>[2x]MPNKYIVVTGGVLSSVGKGTLVASI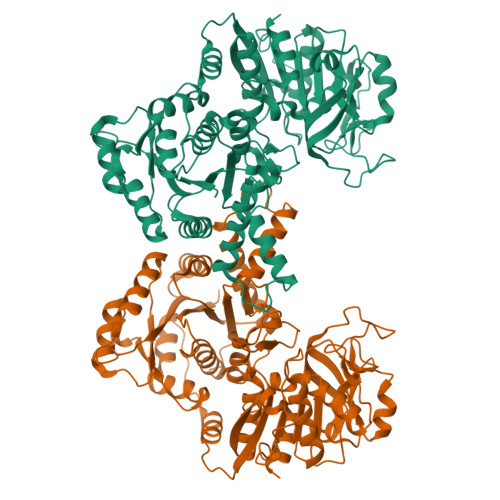GMLLKRRGYNVTAVKIDPYINVDAGTMNPYMHGEVFVTEDGAETDLDLGHYERFMDVNMTKYNNITAGKVYFEVIKKEREGKYLGQTVQIIPHVTDQIKDMIRYASKINNAEITLVEIGGTVGDIESLPFLEAVRQLKLEEGEDNVIFVHIALVEYLSVTGELKTKPLQHSVQELRRIGIQPDFIVGRATLPLDDETRRKIALFTNVKVDHIVSSYDVETSYEVPIILESQKLVSKILSRLKLEDRQVDLTDWISFVNNIKGINSKKTINIALVGKYTKLKDSYISIKEAIYHASAYIGVRPKLIWIESTDLESDTKNLNEILGNVNGIIVLPGFGSRGAEGKIKAIKYAREHNIPFLGICFGFQLSIVEFARDVLGLSEANSTEINPNTKDPVITLLDEQKNVTQLGGTMRLGAQKIILKEGTIAYQLYGKKVVYERHRHRYEVNPKYVDILEDAGLVVSGISENGLVEIIELPSNKFFVATQAHPEFKSRPTNPSPIYLGFIRAVASL> MAAKVFESIGKFGLALAVAGGVVNSALYNVDAGHRAVIFDRFRGVQDIVVGEGTHFLIPWVQKPIIFDCRSRPRNVPVITGSKDLQNVNITLRILFRPVASQL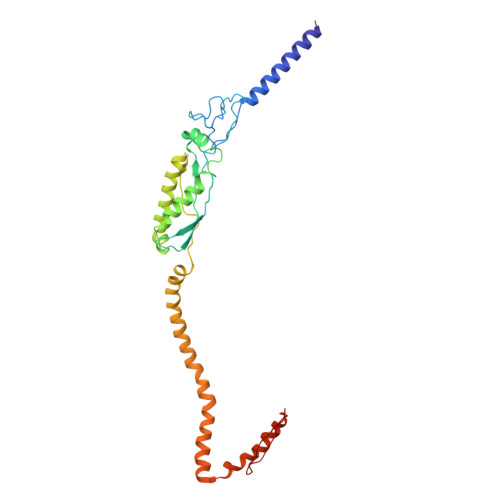PRIFTSIGEDYDERVLPSITTEILKSVVARFDAGELITQRELVSRQVSDDLTERAATFGLILDDVSLTHLTFGKEFTEAVEAKQVAQQEAERARFVVEKAEQQKKAAIISAEGDSKAAELIANSLATAGDGLIELRKLEAAEDIAYQLSRSRNITYLPAGQSVLLQLPQ> SGAGICSLPFLAKICQKIKLAIKNSVPIKDVDSDKYSIFPTLRGYHWRGRDCNDSDKTVYPGRRPDNWDAHRDSNCNGIWGVDPKDGIPYEKKFCEGSQPRGIILLGDAAGAHFHIPPEWLTVSQMSVNSFLNLPTAVTNELDWPQLSGTTGFLDSASKIKENSIYLRLRKRNRCNHRDYQNISKNGASSRNVKSLIESLSRNQLLDHPAIVIYAMIGNDVCNGRKTDPVSAMTTPEQLYANVLKMLEALNSHLPTGSHVILYGLAHGAFLWDTLHSRYHPLGQLNKDVTYTQLYSFLGCLQVSP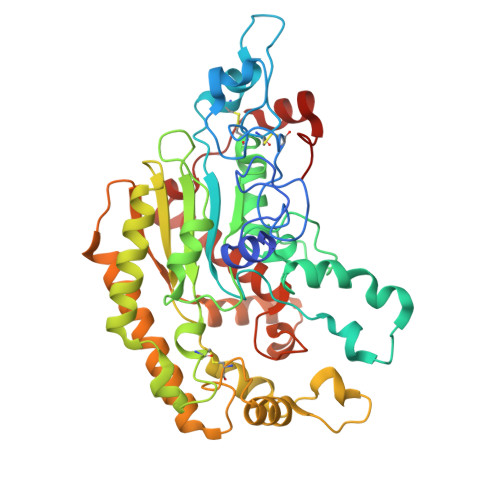CPGWMSANETLRALTSERAQQLSETLRKIAASKKFTNFNLFYLDFAFQEVVEEWQKMGGQPWELIEAVDGFHPNEVALLLFADQLWEKVQRQWPDVLGKENPFNPQIEEVFGDQGGH> MNSDLMLLAAEGARTSTSEAVVFWVVGTVALVGAIGVVAARKAVYSAVFL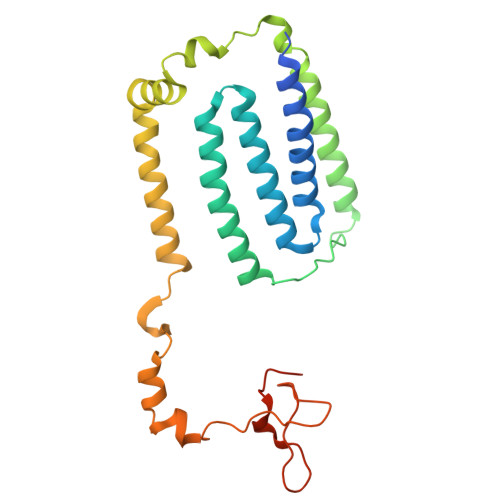ACTMISLAVLYIAQDAPFLGVVQIVVYTGAVMMLFLFVLMLIGVDLTESLVETIKGHRIAALIAGAGFGILVIAGIGNVSVAGFSGLAAANSGGNVEGLAALIFTRYLWAFELTSALLITAALGAMVLAHRERFERRKTQRELAIERFQTGGHPTPLPNPGVYARHNSVDVPARLPDGSESPLSVSTILPHRTVGSATNGKR>MLGNLKPQAPDKILALMGEFRADPRQGKIDLGVGVYKDATGHTPIMRAVHAAEQRMLETETTKTYAGLSGEPEFQKAMGELILGDGLKSETTATLATVGGTGALRQALELARMANPDLRVFVSDPTWPNHVSIMNFMGLPVQTYRYFDAETRGVDFEGMKADLAAAKKGDMVLLHGCCHNPTGANLTLDQWAEIASILEKTGALPLIDLAYQGFGDGLEEDAAGTRLIAS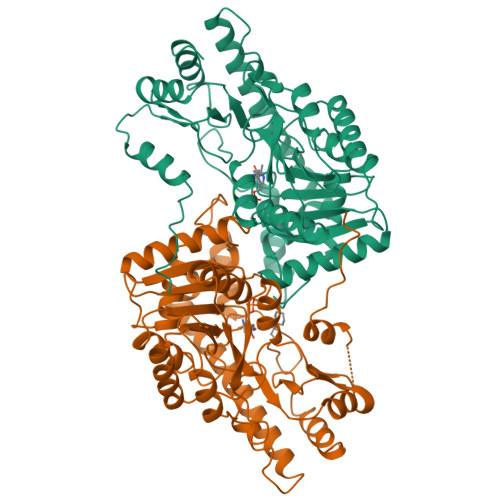RIPEVLIAASCSKNFGIYRERTGCLLALCADAATRELAQGAMAFLNRQTYSFPPFHGAKIVSTVLTTPELRADWMAELEAVRSGMLRLREQLAGELRDLSGSDRFGFVAEHRGMFSRLGATPEQVKRIKEEFGIYMVGDSRINIAGLNDNTIPILARAIIEVGV[2x]>[20x]GSFTMADLDDIKDGKDFRTDQPQKNIPFTLKGCGALDWGMQSRLSRIFNPKTGKTVMLAFDHGYFQGPTTGLERIDINIAPLFEHADVLMCTRGILRSVVPPATNRPVVLRASGANSILAELSNEAVALSMDDAVRLNSCAVAAQVYIGSEYEHQSIKNIIQLVDAGMKVGMPTMAVTGVGKDMVRDQRYFSLATRIAAEMGAQIIKTYYVEKGFERIVAGCPVPIVIAGGKKLPEREALEMCWQAIDQGASGVDMGRNIFQSDHPVAMMKAVQAVVHHNETADRAYELYLSEKQ

While sequence analysis suggests that LsrF will function as a class I aldolase and genetic data suggests LsrF is involved in P-AI-2 processing, the details of the role LsrF plays in processing P-AI-2 are not known. To begin addressing this question, we have determined the crystal structure of LsrF, alone and in complex with the P-AI-2 analogues ribose-5-phosphate and ribulose-5-phosphate. LsrF crystallizes as a decamer with each monomer having an (αβ)8-barrel fold, a ubiquitous fold commonly seen in proteins catalyzing aldolase reactions. The LsrF oligmer has a disk-like structure, with two rings of five monomers stacked on top of each other giving rise to a decamer with D5 symmetry.

To identify the catalytic site of LsrF, we determined the structure of the protein in complex with two P-AI-2 analogues: ribose-5-phosphate (R5P) and ribulose-5-phosphate (5RP). In both structures, the ligand electron density allowed definitive placement of the phosphate group and illustrated the general path of the carbon chain, but was of insufficient quality for unambiguous placement of all ligand atoms. R5P and 5RP bind LsrF in the same location, near the entrance to the (αβ)8-barrel with the phosphate group oriented towards the coils following β7 and β8. The phosphate is located near the positively charged side chain of Arg254 and is positioned to form hydrogen bonds with the side chain of His58, the side chain and main chain of Arg254, and the main chain of three glycine residues: 226, 227, and 253 (in all cases with N or NH groups). The ligand then extends across the center of the (αβ)8-barrel, away from strands 7 and 8, in a largely polar environment. In particular, Lys203 is adjacent to the ligand; this residue has potential significance for the mechanism, as equivalently positioned lysines are responsible for Schiff base formation in other aldolases (below). No large conformational changes were observed upon ligand binding, though there were small movements in a few binding site residues, most notably Asp251 and Met252 (with α-carbons shifting by 0.5–2.0 Å). A single water was built in the binding site of unliganded LsrF; this water is displaced upon ligand binding. The P-AI-2 analogues ribose-5-phosphate and ribulose-5-phosphate bind to LsrF in the same general position that other aldolases bind phosphorylated substrates (e.g. E. coli DERA and FBPA, T. tenax FBPA and M. jannaschii ADH synthase), suggesting that the canonical aldolase active site is conserved in LsrF. Key catalytic residues in these class I aldolases are structurally conserved in LsrF, and both P-AI-2 analogues bind LsrF in the canonical aldolase active site, strongly implicating LsrF as a class I aldolase.> S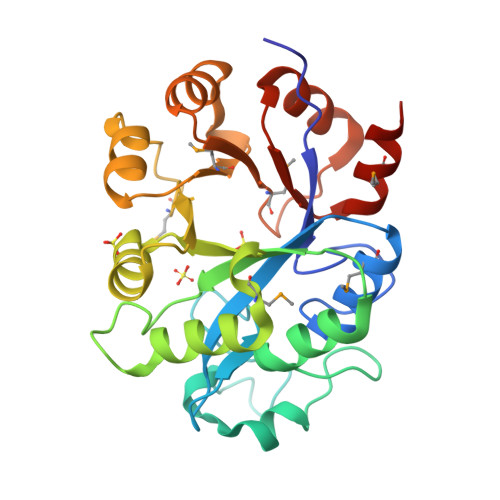SKVIIPKIVGHRGVGKEGLAPENTLRSFVLCMERNIPYIETDLRVCKTGEIVLFHGTPEGTIPFYKDGTSRIGDLSLEELKRLDVGGGHTIPSLEELFVAIEEQKFNLKLNLELKGEEWKRKESGDHQRLLLLVEKYHMQERVDYCSFHHEALAHLKALCPDVKITYLFNYMGQPTPLDFVEQACYGDANGVSMLFHYLTKEQVCTAHEKGLSVTVWMPWIFDDSEEDWKKCLELQVDLICSNYPFGLMNFLSNISE>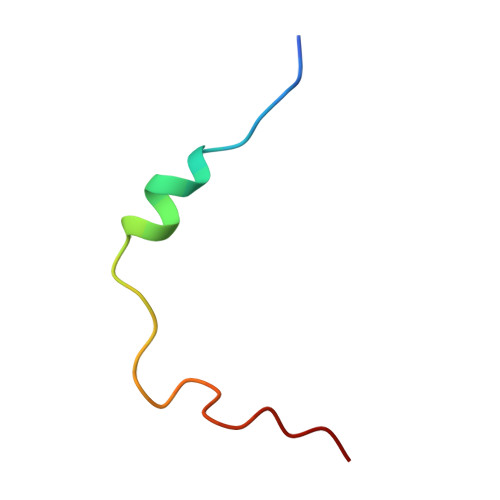 IITPVGESWDSWFDGEGASTDFMSTREQP> MIPHSWICEKHILWLKDYKNSSNWKLFKECWKQGQPAVVSGVHKKMNISLWKAESISLDFGDHQADLLNCKDSIISNANVKEFWDGFEEVSKRQKNKSGETVVLKLKDWPSGEDFKTMMPARYEDLLKSLPLPEYCNPEGKFNLASHLPGFFVRPDLGPRLCSAYGVVAAKDHDIGTTNLHIEVSDVVNILVYVGIAKGNGILSKAGILKKFEEEDLDDILRKRLKDSSEIPGALWHIYAGKDVDKIREFLQKISKEQGLEVLPEHDPIRDQSWYVNKKLRQRLLEEYGVRTCTLIQFLGDAIVLPAGALHQVQNFHSCIQVTEDFVSPEHLVESFHLTQELRLLAENLYFQ;> MIPHSWICEKHILWLKDYKNSSNWKLFKECWKQGQPAVVSGVHKKM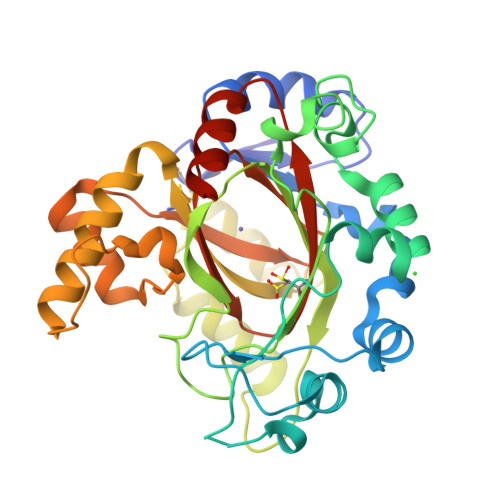NISLWKAESISLDFGDHQADLLNCKDSIISNANVKEFWDGFEEVSKRQKNKSGETVVLKLKDWPSGEDFKTMMPARYEDLLKSLPLPEYCNPEGKFNLASHLPGFFVRPDLGPRLCSAYGVVAAKDHDIGTTNLHIEVDDVVNILVYVGIAKGNGILSKAGILKKFEEEDLDDILRKRLKDSSEIPGALWHIYAGKDVDKIREFLQKISKEQGLEVLPEHDPIRDQSWYVNKKLRQRLLEEYGVRTCTLIQFLGDAIVLPAGALHQVQNFHSCIQVTEDFVSPEHLVESFHLTQELRLLAENLYFQ N-[(1S,2R)-1-benzyl-3-{[(1S)-2-(cyclohexylamino)-1-methyl-2-oxoethyl]amino}-2-hydroxypropyl]-3-(2-oxo-2,3-dihydro-1H-pyrrol-1-yl)-5-propoxybenzamide 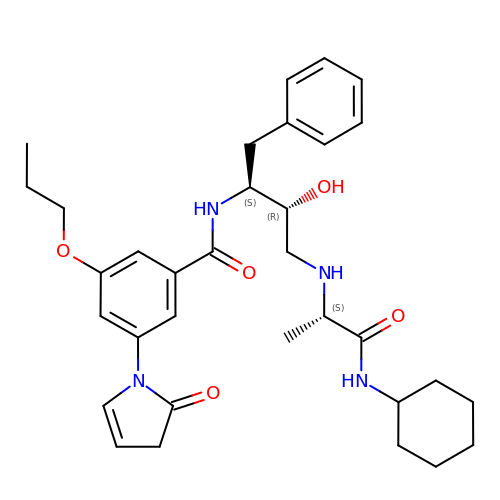| C33 H44 N4 O5 | OCMGZBXBWVXWRJ-KEPSJGTLSA-N>[2x]MVMIDLYTAATPNGHKVS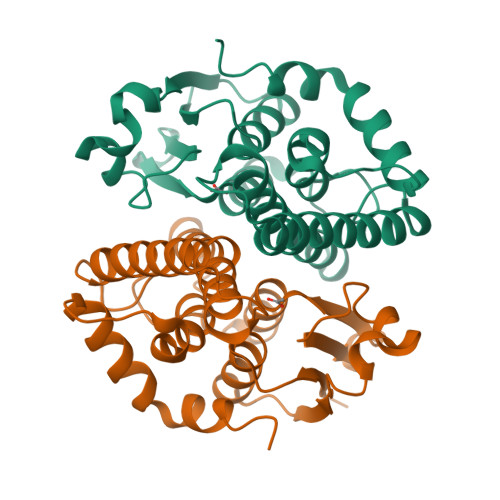IALEEMGLPYRVHALSFDKKEQKAPEFLRINPNGRIPAIVDRDNDDFAVFESGAILIYLAEKTGQLMPADVKGRSRVIQWLMFQMGGVGPMQGQANVFFRYFPEKLQGAIDRYQHETRRLYEVLDGRLGEAEYLAGDYSIADIATYPWVRIHDWSGVAVDGLDNLQRWIAAIEARPAVQRGLLVPRREKEGDDAIRTAQSMLTRAENLYFQSHHHHHHWSHPQFEK>GSMGKDEALEKDLNDVSKEINLMLSTYAKLLSERAAVDASYIDEIDELFKEANAIENALIQKREELRQRFTAIANTLHR[2x]

Meiosis protein TEX12 is an essential component of the synaptonemal complex (SC), which mediates homologous chromosome synapsis. It is also recruited to centrosomes in meiosis, and aberrantly in certain cancers, leading to centrosome dysfunction. Within the SC, TEX12 forms an intertwined complex with SYCE2 that undergoes fibrous assembly, driven by TEX12’s C-terminal tip. TEX12 undergoes conformational change upon C-terminal tip mutations, indicating that the sequence responsible for driving SYCE2-TEX12 assembly within the SC also controls the oligomeric state and conformation of isolated TEX12.

We obtained two distinct crystal forms of TEX12 FFV. Similar to the dimer interface of the ΔCtip tetramer, the FFV structure contains a central ‘hinge’ characterised by reciprocal salt bridges between R78 and D82 amino-acids. Accordingly, the FFV structure matches the symmetry-related dimer (r.m.s. deviation = 1.11 Å) but not the unique chain dimer (r.m.s. deviation = 4.25 Å) of the ΔCtip structure, hence our designation of the former as the dimer interface. FFV’s Ctip sequences play no role in stabilising the dimeric coiled-coil, and simply emanate from either end of the molecule, where they mediate interactions within the crystal lattice. Ctip sequences arrange molecules in an end-on ‘dimer-of-dimers’ fashion by forming inter-molecular anti-parallel coiled-coils. Further, the hydrophobic surface of each Ctip dimer binds to the free Ctip ends of two additional ‘dimer-of-dimers’, forming Ctip tetramers. Given that TEX12 FFV is a stable tetramer in solution, its dimeric crystal structure likely represents an alternative conformation induced by crystallisation. Specifically, the extensive Ctip interactions of the crystal lattice may be mutually exclusive with interactions required for stabilisation of the solution tetramer. The most fundamental unit is formed by the dimer interface, which involves anti-parallel coiled-coil interactions surrounding a central R78-D82 salt bridge hinge, and is the sole interface within the FFV dimer crystal structure.> SMNPPAGPVRAIAEYERSAAVLVRYPFGIPMELIKELAKNDKVITIVASESQKNTVITQYTQSGVNLSNCDFIIAKTDSYWTRDYTGWFAMYDTNKVGLVDFIYNRPRPNDDEFPKYEAQYLGIEMFGMKLKQTGGNYMTDGYGSAVQSHIAYTENSSLSQAQVNQKMKDYLGITHHDVVQDPNGEYINHVDCWGKYLAPNKILIRKVPDNHPQHQALEDMAAYFAAQTCAWGTKYEVYRALATNEQPYTNSLI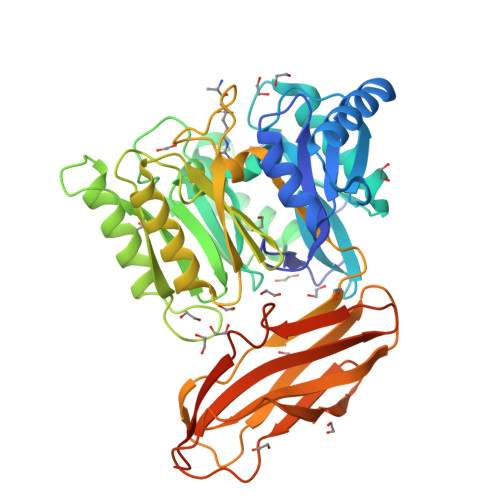LNNRVFVPVNGPASVDNDALNVYKTAMPGYEIIGVKGASGTPWLGTDALHARTHEVADKGYLYIKHYPILGEQAGPDYKIEADVVSCANATISPVQCYYRINGSGSFKAADMTMESTGHYTYSFTGLNKNDKVEYYISAADNSGRKETYPFIGEPDPFKFTCMNETNTCTVTGAAKALRAWFNA>[2x]HHHHHHPCCSNPCQNRGECMSTGFDQYKCDCTRTGFYGENCTTPEFLTRIKLLLKPTPNTVHYILTHFKGVWNIVNNIPFLRSLIMKYVLTSRSYLIDSPPTYNVHYGYKSWEAFSNLSYYTRALPPVADDCPTPMGVKGNKELPDSKEVLEKVLLRREFIPDPQGSNMMFAFFAQHFTHQFFKTDHKRGPGFTRGLGHGVDLNHIYGETLDRQHKLRLF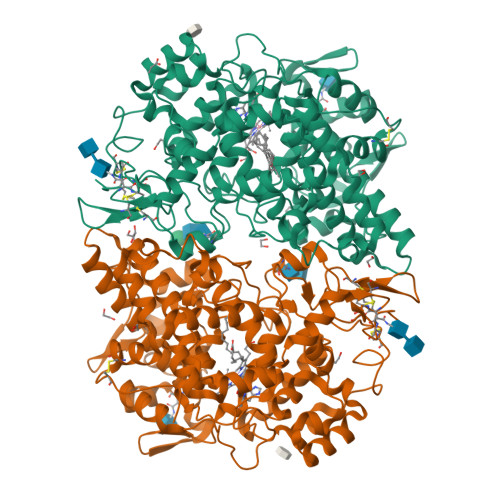KDGKLKYQVIGGEVYPPTVKDTQVEMIYPPHIPENLQFAVGQEVFGLVPGLMMYATIWLREHNRVCDILKQEHPEWGDEQLFQTSRLILIGETIKIVIEDYVQHLSGYHFKLKFDPELLFNQQFQYQNRIASEFNTLYHWHPLLPDTFNIEDQEYSFKQFLYNNSILLEHGLTQFVESFTRQIAGRVAGGRNVPIAVQAVAKASIDQSREMKYQSLNEYRKRFSLKPYTSFEELTGEKEMAAELKALYSDIDVMELYPALLVEKPRPDAIFGETMVELGAPFSLKGLMGNPICSPQYWKPSTFGGEVGFKIINTASIQSLICNNVKGCPFTSFNVQDPQPTKTATIAASASHSRLDDINPTVLIKRRSTEL4-[4-(4-aminophenyl)buta-1,3-diyn-1-yl]-N-[(2S,3S)-4,4-difluoro-3-hydroxy-1-(hydroxyamino)-3-methyl-1-oxobutan-2-yl]benzamide | 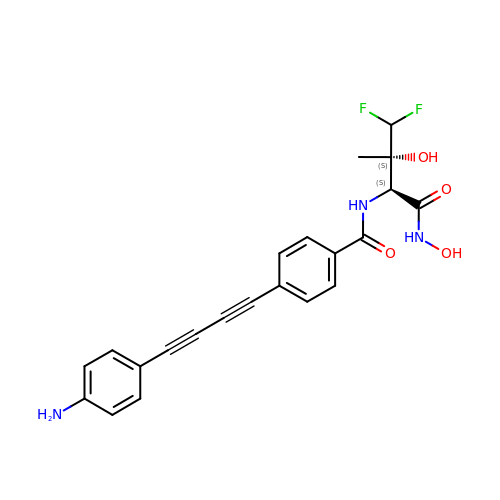C22 H19 F2 N3 O4 | HJOKUNVOXGDMLS-GCJKJVERSA-N> RIIQITRGDSTITSQDVANAIVAYGVWPHYLSSKDASAIDKPSQPDTSSNRFYTLRSVTWSSSSKGWWWKLPDALKDMGIFGENMFYHYLGRSGYTIHVQCNASKFHQGTLIVALIPEHQIASALHGNVNVGYNYTHPGETGREVKAETRLNPDLQPTEEYWLNFDGTLLGNITIFPHQFINLRSNNSA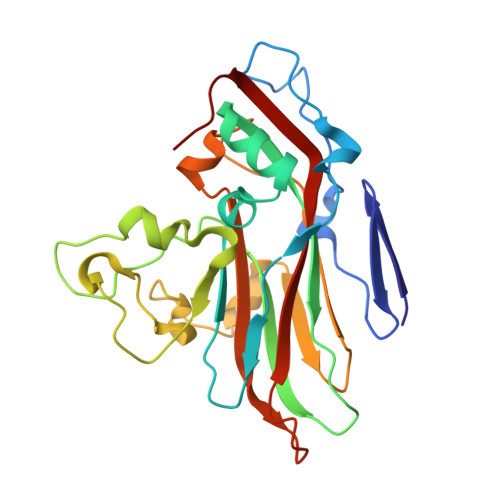TIIAPYVNAVPMDSMRSHNNWSLVIIPICPLETSSAINTIPITISISPMCAEFSGARAKRQ> GPGRAAPPAIREPN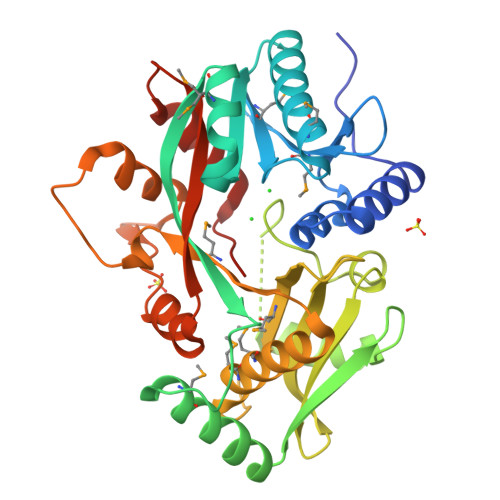AEELQRAARIIRHSDQPDGGLALTGDKALLFHESDDAFLMYARRGRSMIALYDPIGPAMQRAELIWQFRDLCDLHHARPVFYQVRAENLPFYMDIGLTALKLGEEARVDLLRFDLENAGAAMKDLRYTWNRGQRDGLALEFHEPGQAPLDELKAISDAWLGGKQVREKGFSLGRFTPAYLNFFRIAIVRHQGKPVAFANLLETDSRELASLDLMRVHPDAPKLTMEFLMLGLILHYKAQGHARFSLGMVPLAGLQPRRGAPLTQRLGALVFRRGEQFYNFQGLRRFKDKFQPDWEPRYLAVPAGLDPLVALADTAALIAGGLTGLVKR>[2x]MRVLLIHSDYIEYEVKDKALKNPEPISEDMKRGRMEEVLVAFISVEKVDEKNPEEVSLKAIEEISKVAEQVKAENVFVYPFAHLSSELAKPSVAMDILNRVYQGLKERGFNVGKAPFGYYMAFKISCKGHPLAELSRTIVPEEARVE

We have been interested in a D-aminoacyl-tRNA deacylase (DTD) fold that is present across the domains of life in two different functional contexts: as an N-terminal editing domain (NTD) of archaeal ThrRS, which specifically removes non-cognate L-serine mischarged on tRNAThr, and as a freestanding ‘chiral proofreading' enzyme, which removes D-amino acids from tRNAs in bacteria and eukaryotes. Both share a striking structural and mechanistic similarity highlighting a common ancestry. Here we show, with the help of structural, biochemical and biophysical studies from three distant organisms, that the substrate specificity in this domain is determined by a differential remodelling of the catalytic centre at the RNA–protein interface rather than just the presence or absence of catalytic water as previously proposed. While demonstrating that the tRNA provides the catalytic group, we show that the side chains within the recognition site are dispensable for the proofreading function, suggesting a primordial mode of protein- or peptide scaffold-based enzymatic activity evolved alongside that of RNA.

On the other hand, the Lys to Met mutant, although showed partial activity against L-Ser-(Ec)tRNAThr in our earlier work, in subsequent studies with not only PabNTD K121M but also the corresponding K116M and K122M mutants of ApNTD and MjNTD with multiple batches of protein showed a severely compromised activity, suggesting a crucial role of this residue in enzyme function. However, a direct role of Lys in catalysis is still highly unlikely considering that this position is naturally occupied by a Met in the structural homologue DTD. We solved the crystal structure of K121M mutant of PabNTD and K116M mutant of ApNTD with L-Ser3AA and L-Thr3AA to investigate the structural basis of the observed loss of activity. A significant repositioning of the crucial catalytic water was observed upon mutation of the polar Lys side chain to the non-polar Met side chain, which is present in DTD. This provides a clear structural basis for the loss of function in this mutant, despite its high binding affinity for the substrate. Therefore, we show that Lys plays a crucial role in positioning the water molecule for catalysis rather than acting as a nucleophile.> MTSEQTGEPAEDTSGVIKMAVKFDRRAYPAQ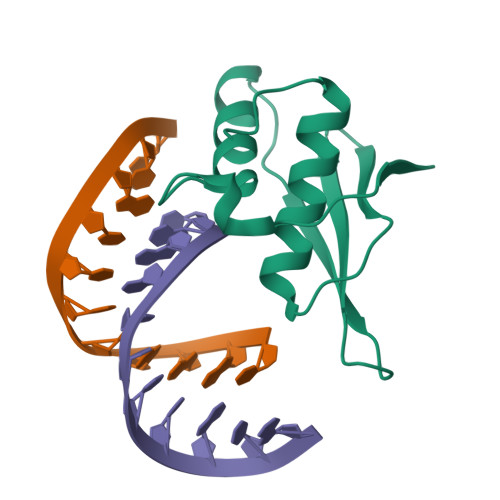ITPKMCLLEWCRREKLAQPVYETVQRPLDRLFSSIVTVAEQKYQSTLWDKSKKLAEQAAAIVCLRSQGLPEGRLGEESPSLHKHHHHHH>YFQSNAMAKSEGKVNGATLMARALQQQGVQYMFGIVGFPVIPIAIAAQREGITYIGMRNEQSASYAAQAASYLTGRPQACLVVSGPGVVHALAGLANAQVNCWPMLLIGGASAIEQNGMGAFQEERQVLLASPLCKYAHQVERPERIPYYVEQAVRSALFGRPGAAYLDMPDDVILGEVEEAAVRPAATVGEPPRSLAPQENIEAALDALQSAKRPLVIVGKGMAWSRAENEVRQFIERTRLPFLATPMGKGVMPDDHPLSVGGARSHALQEADLVFLLGARFNWILHFGLPPRYSKDVRVIQLDLSAEEIGNNRQAEVALVGDGKAIVGQLNQALSSRQWFYPAETPWREAIAAKIAGNQAAVAPMIADNTSPMNYYRVYRDIAARLPRNAIIVGEGANTMDIGRTQMPNFEPRSRLDAGSYGTMGIGLGFAVAAAAVHPGRPVIAVQGDSAFGFSGMEFETAARYGMPIKVIILNNGGIGMGSPAPRDGQPGMPHALSHDARYERIAEAFGGAGFYVTDSAELGPALDAAMAFKGPAIVNIKIAATADRKPQQFNWHG[4x]

One such enzyme is 2-hydroxyacyl-CoA lyase/synthase (HACL/S), which catalyzes the reversible cleavage of 2-hydroxyacyl-CoA (2hcCoA) into formyl-CoA (fCoA) and an aldehyde or ketone. Originally identified in the mammalian α-oxidation pathway of 3-methyl-branched fatty acids, HACL/S has demonstrated remarkable catalytic reversibility, as it is capable of condensing fCoA with various substrates covering a wide range of aldehydes and ketones with different carbon chain lengths. All the enzymes are tetramers, specifically dimers of dimers (α2), where α2 dimer represents a catalytical unit. The three domains have specific functions: the N-terminal domain binds the pyrimidine of ThDP (PYR), the middle domain has a regulatory function (R) and binds ADP, and the C-terminal domain binds the pyrophosphoryl group (PP) of ThDP.

Of particular interest here are the structures of ApbHACL/S with fCoA and D-/L-lCoA. The structure of ApbHACL/S with L-lCoA shows a partly ordered acyl with a clearly visible sulfur atom. ApbHACL/S yielded the structures with CoA-ThDP and ThDP-hmCoA, as well as complexes with acetaldehyde, fCoA, L-lCoA and D-lCoA. However, in several our structures of ApbHACL/S and TbHACL/S with CoA derivatives we observe states where acyl-CoA is no longer connected to ThDP, as the sulfur-carbon bond (S-C2 in acyl-CoA) is broken. These may correspond to post reaction states. In addition, three structures contain covalent adducts to ThDP (“oxo-ThDP” and “hydroxymethyl-ThDP”). In these structures “=O” atom or “-C–O” moiety remain attached to C2 of the thiazolium ring. We suggest these “oxo-ThDP” and “hydroxymethyl-ThDP” adducts to be products of off pathway reactions. Based on the kinetic characterization ApbHACL/S, DhcHACL/S and TbHACL/S are the top three variants that showed the highest catalytic efficiency toward acetaldehyde. This may explain why only these three variants are fully resolved in complex with ligands when lactyl-CoA was co-crystalized as a substrate.>GQRAVALYDFEPENDNELRLAEGDIVFIS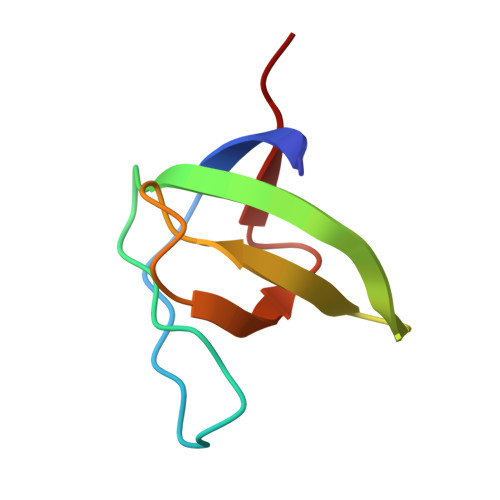YKHGQGWLVAENESGSKTGLVPEEFVSYIQ[6x]>[6x]MTDMSIKFELIDVPIPQGTNVIIGQAHFIKTVEDLYEALVTSVPGVKFGIAFCEASGKRLVRHEANDEELRNLAIDLCK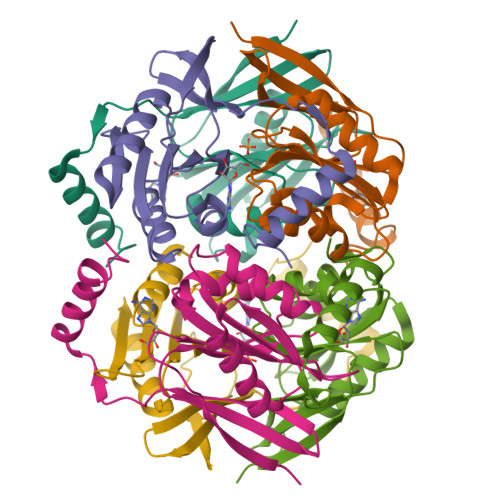KIAAGHVFVIYIRNAWPINVLNAIKNVPEVVRIFAATANPLKVIVAEVEPERRGVVGVVDGHSPLGVETEKDREERKKFLREVVKYKL>HMDKDKTVV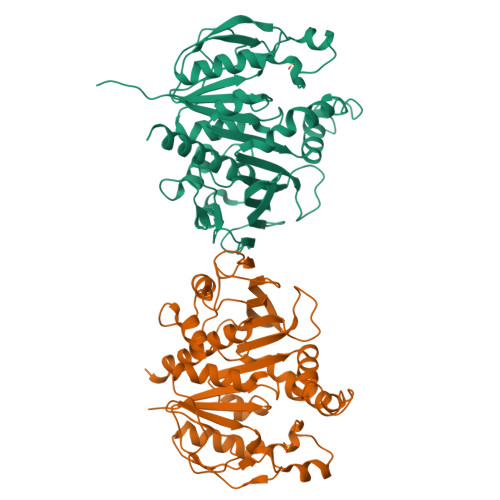IGLAADSGCGKSTFMRRMTSIFGGVPKPPAGGNPDSNTLISDMTTVICLDDYHCLDRNGRKVKGVTALAPEAQNFDLMYNQVKALKEGKSVDKPIYNHVSGLIDAPEKIESPPILVIEGLHPFYDKRVAELLDFKIYLDISDDIKFAWKIQRDMAERGHSLESIKSSIAARKPDFDAYIDPQKKDADMIIQVLPTQLVPDDKGQYLRVRLIMKEGSKMFDPVYLFDEGSTISWIPCGRKLTCSFPGIKMFYGPDTWYGQEVSVLEMDGQFDKLEELIYVESHLSNTSAKFYGEITQQMLKNSGFPGSNNGTGLFQTIVGLKVREVYERIVKKDVVPV[2x]>[4x]RRFGYAIVGLGKYALNQILPGFAGCQHSRIEALVDGNAEKAKIVAAEYGVDPRKIYDYSNFDKIAKDPKIDAVYIILPNSLHAEFAIRAFKAGKHVMCEKPMATSVADCQRMID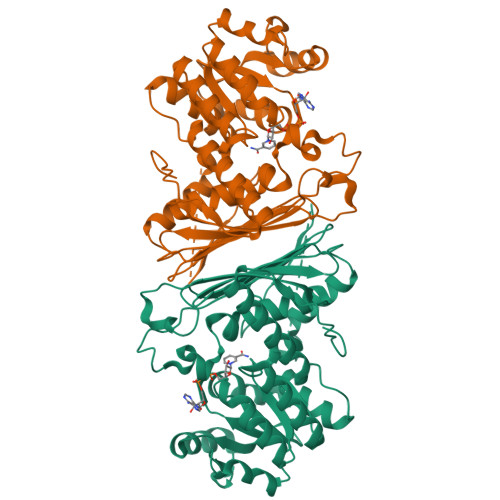AAKAANKKLMIGYRCHYDPMNRAAVKLIRENQLGKLGMVTTDNSDVMDQNDPAQQWRLRRELAGGGSLMDIGIYGLNGTRYLLGEEPIEVRAYTYSDPNDERFVEVEDRIIWQMRFRSGALSHGASSYSTTTTSRFSVQGDKAVLLMDPATGYYQNLISVQTPGHANQSMMPQFIMPANNQFSAQLDHLAEAVINNKPVRSPGEEGMQDVRLIQAIYEAARTGRPVNTDWGYVRQGGY>[4x]GSHMARYDSLLQALGNTPLVGLQRLSPRWDDGRDGPHVRLWAKLEDRNPTGSIKDRPAVRMIEQAEADGLLRPGATILEPTSGNTGISLAMAARLKGYRLICVMPENTSVERRQLLELYGAQIIFSAAEGGSNTAVATAKELAATNPSWVMLYQYGNPANTDSHYCGTGPE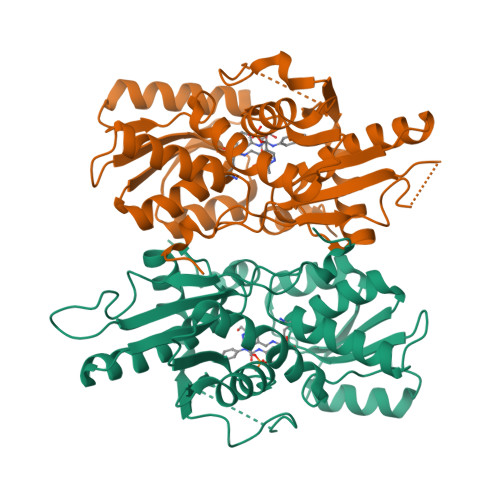LLADLPEITHFVAGLGTTGTLMGTGRFLREHVANVKIVAAEPRYGEGVYALRNMDEGFVPELYDPEILTARYSVGAVDAVRRTRELVHTEGIFAGISTGAVLHAALGVGAGALAAGERADIALVVADAGWKYLSTGAYAGSLDDAETALEGQLWA>[4x]MNHKVHHHHHH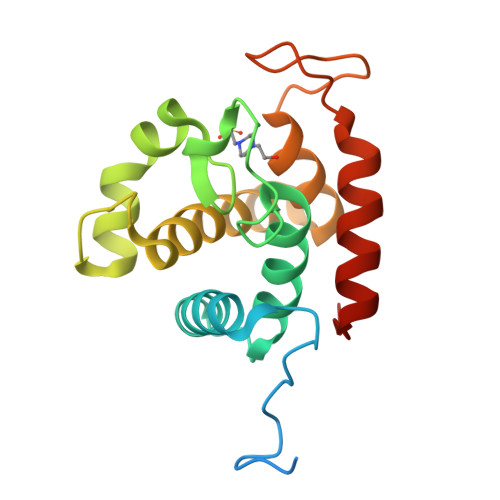IEGRHMGTTPSDPPTNPPTTVTKPAEVPSRIWTYVMNADNAYGKGGDFALLLSAVIKKESYFGDGLSGSPSAGDGLMQVQPNTRNAYLSQFSAKYGHAYNHSSEQDQVYMGSLILNEKIVRFGSIYSGLLHYNGGDYWYPGATDSYGRPILADQYANTVYAQYKSYGGRYSR> GMSNALATLASPADDIAFYEERLRAAMLTGDLKGLETLLADDLAFVDHTGCVKTKQTHL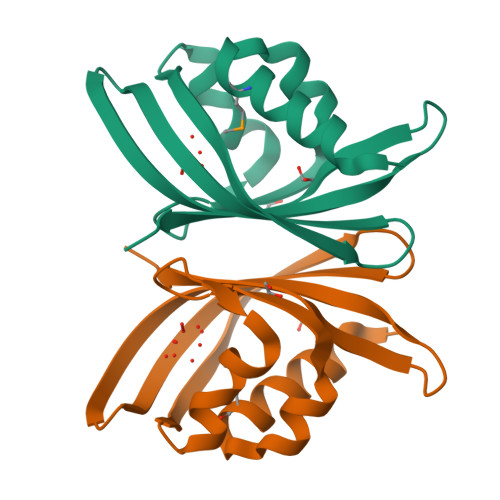EPYRAGLLKLSRLDLSDAVVRAAGEDGRVVVVRAVTAGVYDGEAFTETLRFTRIWRRTQGPAGWKLVAGHCSVIL> GHPTLKTPESVTGTWKGDVKIQCIYDPLRGYRQVLVKWLVRHGSDSVTIFLRDSTGDHIQQAKYRGRLKVSHKVPGDVSLQINTLQMDDRN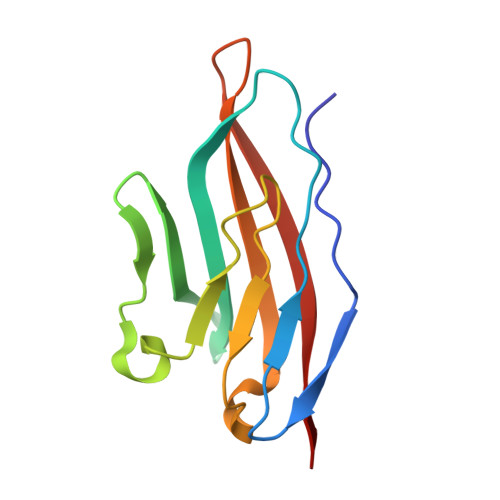HYTCEVTWQTPDGNQVIRDKIIELRVRK>[4x]MADLNWISSALIKERPSADAVLAKAVLAAREQLGLTQLELAGIVGVDRSAISRWKTQGLRVDSKTGELALLLVRVYRALYALFGGQQEDMRHFLRTPNHHLAGEPLALMGQVQGLVHVLEYLDAIRGKV;>MGSSHHHHHHSQDPSEIWRQCKGERHIRPLQGRLVRLVESQEQVATLQLVDTLEEQALLEELLESSKPPVPADAEPLHYLL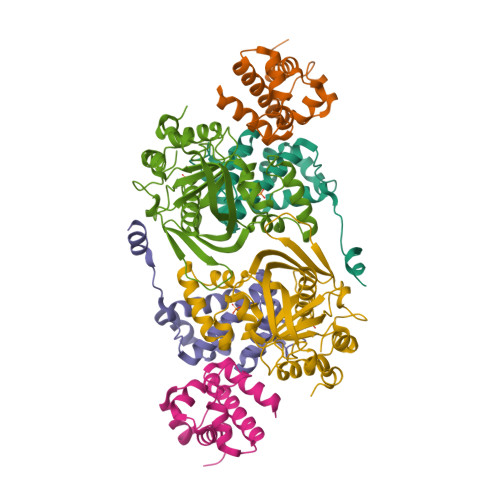KTPFRYPPLRWGSRFGRRHEPSLFYAALKLETAMAESAYYRCVLWSGMVVPPPSGRILSEHASFEAGWKVERGIRLQAPPFSDHEAALTDIADYRAPQELGSAMRSAGVQAFEYRSARCPERGCNVALFTPAAFTEKRPRNLTPWLCETTAGYVAFKPAHVPGSPKIFSWELFLVDGKLPHPA[2x]Even in simple eukaryotes like yeast and amoebazoa, myosin I exists in several isoforms, which carry out distinct functions but the genome of E. histolytica has a single isoform of myosin I, namely EhMyosin IB. EhMyosin IB has been observed to localize in phagocytic cups during erythrophagocytic processes. The SH3 domain located in the tail region of myosin I plays a prominent role in bridging the processes of actin assembly and endocytosis. In the current work, we have identified a novel interaction between the SH3 domain of unconventional EhMyosin IB and the c-terminal domain of EhFP10, and showed this interaction to regulate the phagocytic and pinocytic processes by affecting the cytoskeletal dynamics.

In a previous study, EhMySH3 was predicted to preferentially bind pseudo-symmetrical and class II ligands. Chosen ligands belonged to class I (P4), class II (P1), and an overlapping pseudo-symmetrical sequence belonging to both classes (P2), as predicted by “SH3 HUNTER’ software. The results showed that the P2 peptide, with a pseudosymmetrical ligand (overlapping class I and class II motif) from EhFP10 displayed highest binding response relative to other peptides, as was predicted in our previous study. We were able to crystallize EhMySH3 in complex with the pseudo-symmetrical peptide P2 [KVAPPIPHR]. Peptide, P2 is located between 653–661 residues in the c-terminal domain of the EhFP10 molecule. The EhMYSH3-P2 complex crystallized with two molecules of EhMySH3 and one P2 peptide per asymmetric unit, and with P2 binding to chain A of one EhMySH3 molecule and chain B of a symmetry-related EhMySH3 molecule. P2 was observed to make more electrostatic interactions with chain B than with chain A. P2 binds to EhMySH3 chain B in class II pattern, i.e., [xPxxPx(K/R)]. P2 residues A3 and P4 formed the first XP motif, which fit in the first consensus hydrophobic pocket made by residues Y9 and Y52 of EhMySH3; and I5 and P6 formed the second XP motif, which occupied the second hydrophobic pocket made by residues P49 and W36 of EhMySH3. The c-terminal residue R9 of P2 was observed to interact with residue E34 of the n-Src loop present in the specificity pocket of EhMySH3. In our case, though the electron density for the terminal R9 residue was not complete, after refinement we obtained better electron density near the n-Src loop, though there could be an alternate conformation near E18 in the RT loop, likely to be one of the probable orientations for residue R9.

>[2x]MSKLPQVKALYPYTAANDEELSFKVGDIITILEKDEGWWKGELNGQEGWIPNNYVKEILEHHHHHH;> KVAPPIPHR>[2x]MSMEEEEFDIREALANGEHLEKILIMAKYDESVLKKLIELLDDDLWTVVKNAISIIMVIAKTREDLYEPMLKKLFSLLKKSEAIPLTQEIAKAFGQMAKEKPELVKSMIPVLFANYRIGDEKTKINVSYALEEIAKANPMLMASIVRDFMSMLSSKNREDKLTALNFIEAMGENSFKYVNPFLPRIINLLHDGDEIVRA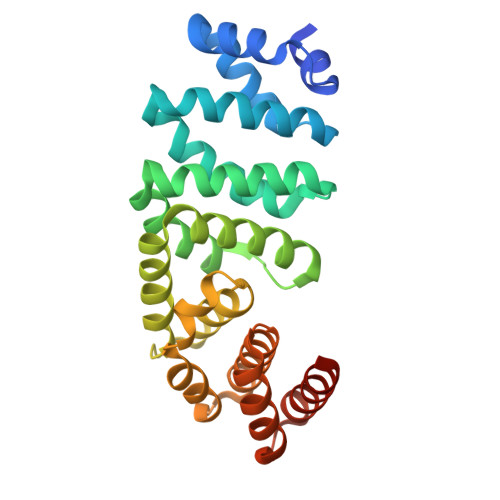SAVEALVHLATLNDKLRKVVIKRLEELNDTSSLVNKTVKEGISRLLLLEGHSSS>GSFVGSIDQGTTSSRFLIFNGEGNPVASHQIEFENLYPKSGWHEQDPYELLNSVQQCIDGAMHKFASLGYSKENIRAIGITNQRETTVVWDSVTGEPLHNAIVWPDTRTSALVRELKARQSADSLLELCGLPLSTYPSSVKLLWLIQNVDAVKQAYEEGRLAFGTVDSWLIYKLNGGAQAERPIHVTDSTNASRTMFMNLRTLQYDDKLLGFFGIDRNKIK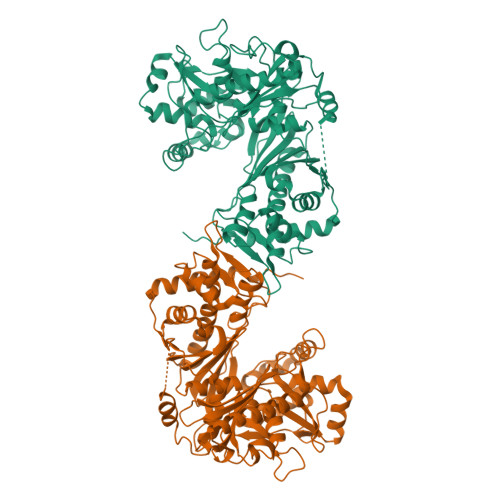LPKIVPSSDPEAFGKVATGALAGVPIAGCLGDQSSALVGQCGFSPGQAKNTYGTGCFLLYNVGTEPVISKYGLLATVAYDFGRGRKPVYALEGSIAVAGAGITFLMNNLGFAPKPSEINALAESVLDNGGVVFVTAFSGLFAPYWIDDAKGTLFGITQHTTKGHIARATLEATCYQTRAILDAMEKDSGHKLESLAVDGGLSASDLCMQTQADISGIPVDRPRMRETTALGAAIAAGLATGVWRELDHVKESIAGGANGNGKKNAREVFYPKMDRKKAERLFRKWEQAVEMSRGWVREQEEEDGE[2x]>[2x]IEKKIVLRNGTEAFDSWEKPPLPVYTQFYFFNVTNPEEILRGETPRVEEVGPYTYRELRNKANIQFGDNGTTISAVSNKAYVFERDQSVGDPKIDLIRTLNIPVLTVIEWSQVHFLREIIEAMLKAYQQKLFVTHTVDELLWGYKDEILSLIHVFRPDISPYFGLFYEKNGTNDGDYVFLTGEDSYLNFTKIVEWNGKT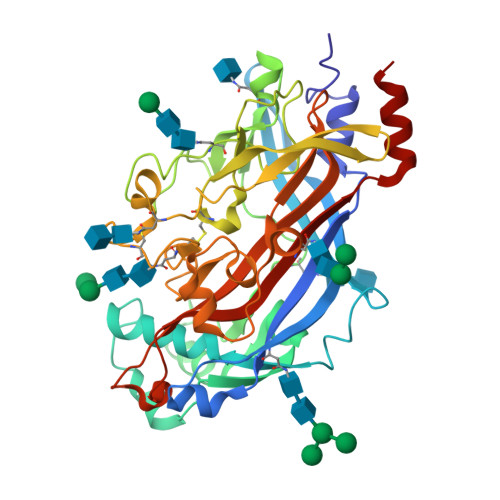SLDWWITDKCNMINGTDGDSFHPLITKDEVLYVFPSDFCRSVYITFSDYESVQGLPAFRYKVPAEILANTSDNAGFCIPEGNCLGSGVLNVSICKNGAPIIMSFPHFYQADERFVSAIEGMHPNQEDHETFVDINPLTGIILKAAKRFQINIYVKKLDDFVETGDIRTMVFPVMYLNESVHIDKETASRLKSMIN> MAHAGRTGYDNREIVMKYIHYKLSQRGYEWDAGDDVEENRTEAPEGTESEVVHLTLRQAGDDFERRYRR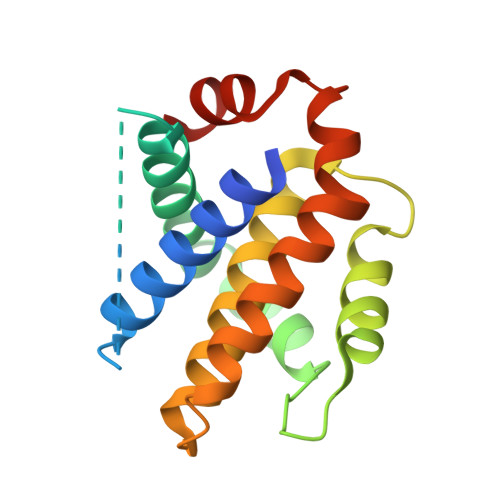DFAEMSSQLHLTPFTARGRFATVVEELFRDGVNWGRIVAFFEFGGVMCVESVNREMSPLVDNIALWMTEYLNRHLHTWIQDNGGWDVFVELYGPSMR>[4x]GCCGGAUGGC

In order to understand the structural basis for the effect of N6‐methyladenine on k‐turn conformation, we have used X‐ray crystallography to investigate the structural effect of this modification on different base pairs involving adenine. Each species was formed by the hybridization of a self‐complementary strand that contains a 5‐bromocytosine nucleotide used to calculate phases for the diffraction in most cases. Crystallography reveals that N6‐methylation of adenine prevents the formation of trans Hoogsteen‐sugar A·G base pairs, explaining why the box C/D RNA cannot adopt its kinked conformation. More generally, our data indicate that sheared A·G base pairs (but not Watson–Crick base pairs) are more susceptible to disruption by N6mA methylation and are therefore possible regulatory sites.

We studied another duplex of sequence identical to that of the previous one, except that the G‐C base pairs flanking the central G·A pairs were replaced by G·U pairs. Two forms were synthesized, with and without N6‐methyladenine replacing the central adenine bases that oppose the guanine nucleotides. In marked contrast, in the N6‐methyladenine‐containing duplex the guanine and N6‐methyladenine do not form base pairs. Superposition shows that it is primarily the N6‐methyladenine that has become displaced, with a large in‐plane translation so that the previously H‐bonded distances are now > 6 Å. This avoids a steric clash between the additional methyl groups and the ribose of the opposing guanine (AN6 is just 3 Å from the ribose in the trans sugar‐Hoogsteen G·A base pair). In its new position, AN6 donates a H‐bond to the O2′ of the opposing G (2.8 Å) and the methyl group is free from steric clash. Note that the G·N6mA base pair is disrupted, such that the N6‐methyladenine is significantly translated away from the opposing guanine base. Thus, the effect of N6‐methylation of adenine in this context is the complete disruption of the trans sugar‐Hoogsteen base pair with guanine and is therefore incompatible with the k‐turn conformation. Thus, N6‐methylation of adenine prevents the formation of the trans Hoogsteen‐sugar G·A base pair.>RSNVFAVDSQIPTLYMPQYISLSGVMTNDGPDNQAIASFEIRDQYITALNHLVLSLELPEVKGMGRFGYVPYVGYKCINHVSISSCNGVIWEIEGEELYNNCINNTIALKHSGYSSELNDISIGLTPNDT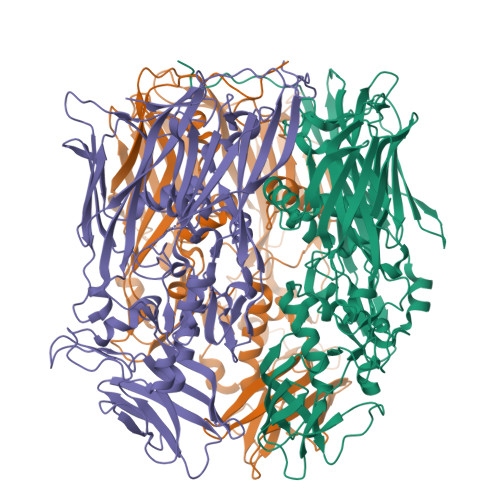IKEPSTVYVYIKTPFDVEDTFSSLKLSDSKITVTVTFNPVSDIVIRDSSFDFETFNKEFVYVPELSFIGYMVKNVQIKPSFIEKPRRVIGQINQPTATVTEVHAATSLSVYTKPYYGNTDNKFISYPGYSQDEKDYIDAYVSRLLDDLVIVSDGPPTGYPESAEIVEVPEDGIVSIQDADVYVKIDNVPDNMSVYLHTNLLMFGTRKNSFIYNISKKFSAITGTYSDATKRTIFAHISHSINIIDTSIPVSLWTSQRNVYNGDNRSAESKAKDLFINDPFIKGIDFKNKTDIISRLEVRFGNDVLYSENGPISRIYNELLTKSNNGTRTLTFNFTPKIFFRPTTITANVSRGKDKLSVRVVYSTMDVNHPIYYVQKQLVVVCNDLYKVSYDQGVSITKIMG[3x]>GSHMLEGGVEVLSVVTGEDSITQIELYLNPRMGVNSPDLPTTSNWYTYTYDLQPKGSSPDQPIKENLPAYSVARVSLPMLNEDITCDTLQMWEAISVKTEVVGISSLINVHYWDMKRVHDYGAGIPVSGVNYHMFAIGGEPLDLQGLVLDYQTQY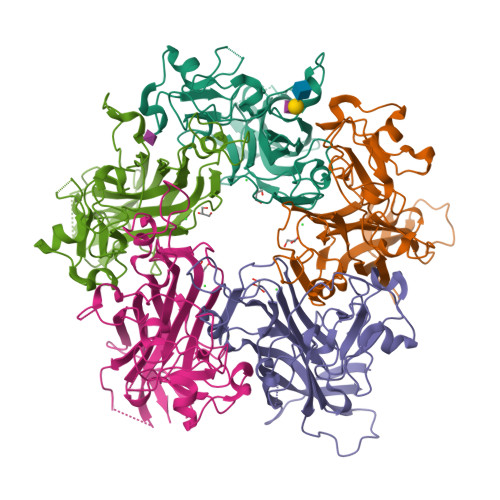PKTTNGGPITIETVLGRKMTPKNQGLDPQAKAKLDKDGNYPIEVWCPDPSKNENSRYYGSIQTGSQTPTVLQFSNTLTTVLLDENGVGPLCKGDGLFISCADIVGFLFKTSGKMALHGLPRYFNVTLRKRWVKN[20x]2-oxopentadecyl-CoA | C36 H64 N7 O17 P3 S | 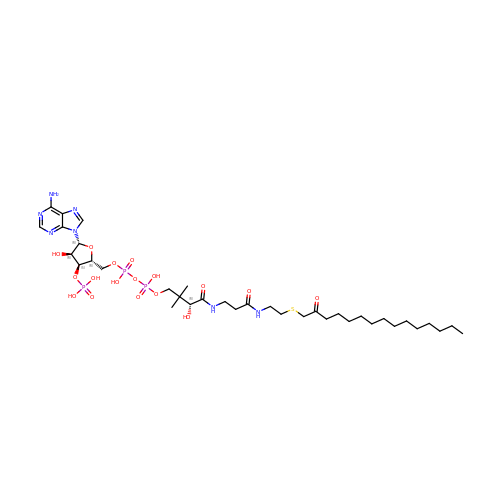JKWHUJMJVNMKEF-UOCZADIYSA-J> MPSYKSSRVLVRDVPEELVDHYERSHRVAAFFMRLLLAMRREPYSLRMR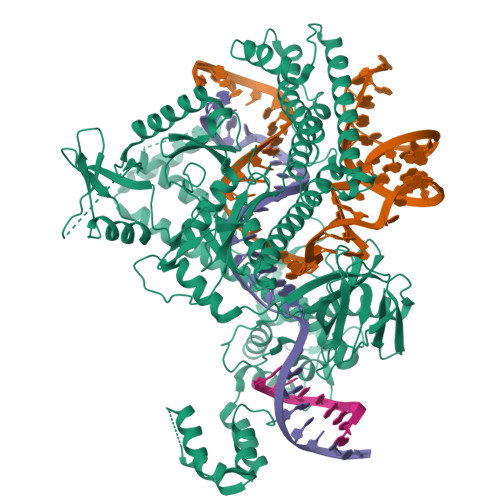DGTEREVDLDETDDFLRSAGCEEPDAVSDDLRSFALAVLHQDNPKKRAFLESENCVSILCLEKSASGTRYYKRPGYQLLKKAIEEEWGWDKFEASLLDERTGEVAEKFAALSMEDWRRFFAARDPDDLGRELLKTDTREGMAAALRLRERGVFPVSVPEHLDLDSLKAAMASAAERLKSWLACNQRAVDEKSELRKRFEEALDGVDPEKYALFEKFAAELQQADYNVTKKLVLAVSAKFPATEPSEFKRGVEILKEDGYKPLWEDFRELGFVYLAERKWERRRGGAAVTLCDADDSPIKVRFGLTGRGRKFVLSAAGSRFLITVKLPCGDVGLTAVPSRYFWNPSVGRTTSNSFRIEFTKRTTENRRYVGEVKEIGLVRQRGRYYFFIDYNFDPEEVSDETKVGRAFFRAPLNESRPKPKDKLTVMGIDLGINPAFAFAVCTLGECQDGIRSPVAKMEDVSFDSTGLRGGIGSQKLHREMHNLSDRCFYGARYIRLSKKLRDRGALNDIEARLLEEKYIPGFRIVHIEDADERRRTVGRTVKEIKQEYKRIRHQFYLRYHTSKRDRTELISAEYFRMLFLVKNLRNLLKSWNRYHWTTGDRERRGGNPDELKSYVRYYNNLRMDTLKKLTCAIVRTAKEHGATLVAMENIQRVDRDDEVKRRKENSLLSLWAPGMVLERVEQELKNEGILAWEVDPRHTSQTSCITDEFGYRSLVAKDTFYFEQDRKIHRIDADVNAAINIARRFLTRYRSLTQLWASLLDDGRYLVNVTRQHERAYLELQTGAPAATLNPTAEASYELVGLSPEEEELAQTRIKRKKREPFYRHEGVWLTREKHREQVHELRNQVLALGNAKIPEIRT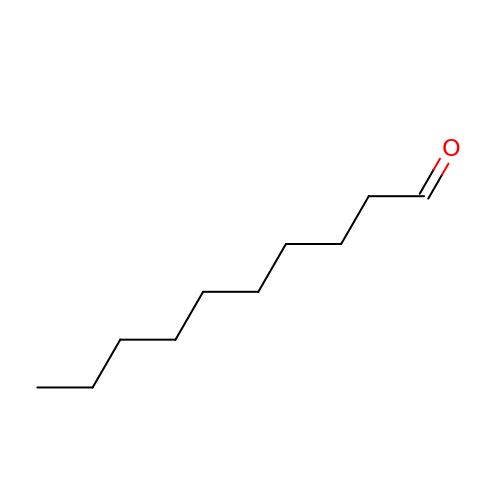decanal | C10 H20 O | KSMVZQYAVGTKIV-UHFFFAOYSA-N>GSGMEVDDRVSALEQRLQLQEDELAVLKAALADALRRLRACEEQGAA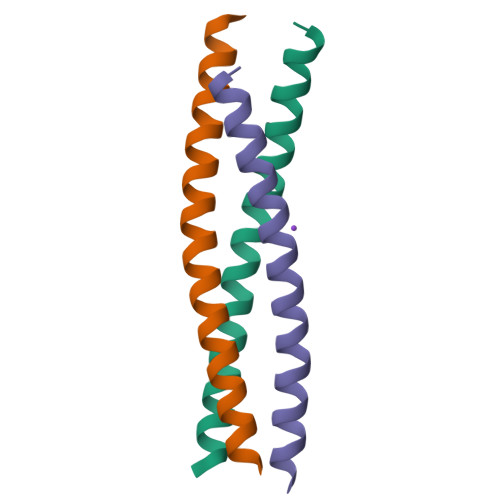LRAR[6x]> GA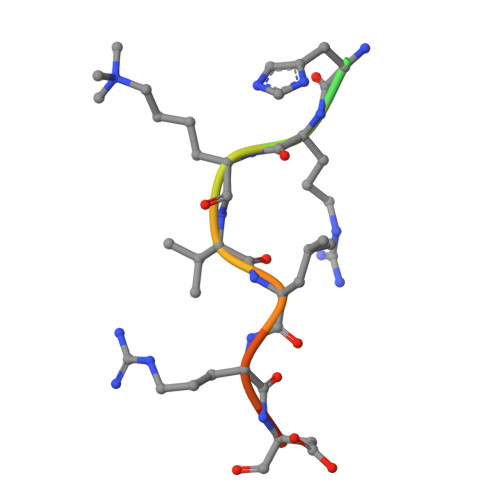KRHRKVLRDNY(3S)-1,3-dihydroxy-4-{[(S)-hydroxy(phosphonooxy)phosphoryl]oxy}-2-methylbut-2-ylium, carbokation intermediate | C5 H13 O9 P2 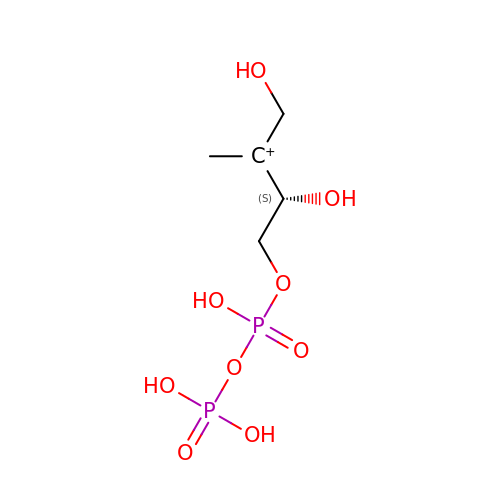| NBNBDNPPGPBHHB-RXMQYKEDSA-O>[8x]MHHHHHHMNPERSERIEIPVLPLRDVVVYPHMVIPLFVGREKSIRCLEAAMDHDKKIMLVAQKEASTDEPGVNDLFTVGTVASILQMLKLPDG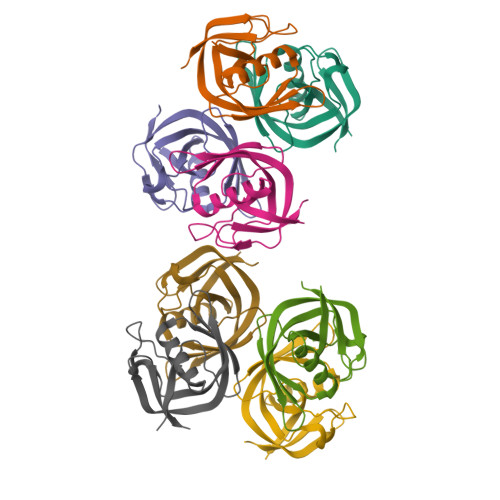TVKVLVEGLQRARISALSDNGEHFSAKAEYLE N-{(2S,3R,4E)-1-[(3,6-di-O-sulfo-beta-D-galactopyranosyl)oxy]-3-hydroxyoctadec-4-en-2-yl}dodecanamide 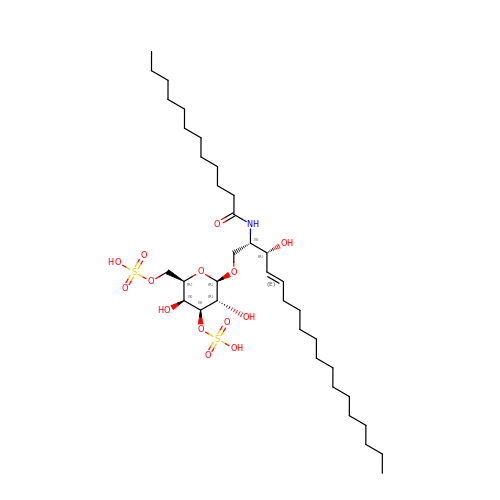| C36 H69 N O14 S2 | JBJSVLZKWGLXMO-AZNTWQPMSA-N> MPLLTQQIQDEDDQYSLVASLDNVRNLSTILKAIHFREHATCFATKNGIKVTVENAKCVQANAFIQAGIFQEFKVQEESVTFRINLTVLLDCLSIFGSSPMPGTLTALRMCYQGYGYPLMLFLEEGGVVTVCKINTQEPEETLDFDFCSTNVINKIILQSEGLREAFSELDMTSE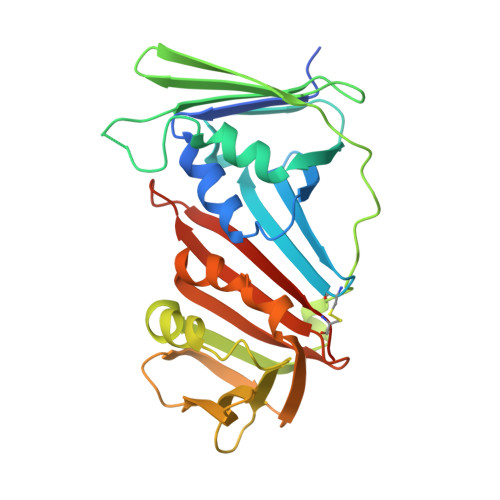VLQITMSPDKPYFRLSTFGNAGSSHLDYPKDSDLMEAFHCNQTQVNRYKISLLKPSTKALVLSCKVSIRTDNRGFLSLQYMIRNEDGQICFVEYYCCPDEEVPESES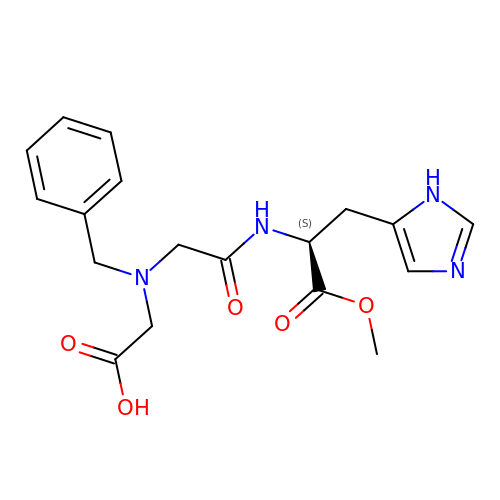2-[[2-[[(2S)-3-(3H-IMIDAZOL-4-YL)-1-METHOXY-1-OXO-PROPAN-2-YL]AMINO]-2-OXO-ETHYL]-(PHENYLMETHYL)AMINO]ETHANOIC ACID | C18 H22 N4 O5 | VJXRDRMNYWCCEG-HNNXBMFYSA-N>MHHHHHHAGNSILLAAVSILSACQQSYFALQVGKARLKYKVTPPAVTGSPEFERVFRAQQNCVEFYPIFIITLWMAGWY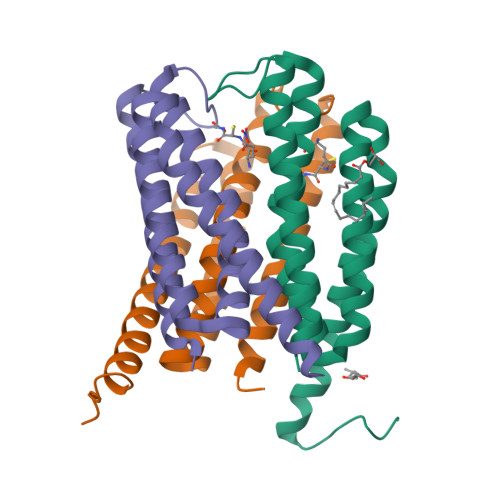FNQVFATCLGLVYIYGRHLYFWGYSEAAKKRITGFRLSLGILALLTLLGALGIANSFLDEYLDLNIAKKLRRQF[3x]> MSQEALKAPVVVLGAGLASVSFVAELRQAGYQGLITVVGDEAERPYDRPPLSKDFMAHGDAEKIRLDCKRAPEVEWLLGVTAQSFDPQAHTVALSDGRTLPYGTLVLATGAAPRALPTLQGATMPVHTLRTLEDARRIQAGLRPQSRLLIVGGGVIGLELAATARTAGVHVSLVQTKPRLMSRAAPATLADFVARYHAAQGVDLRFERSVTGSVDGVVLLDDGTRIAADMVVVGIGVLANDALARAAGLACDDGIFVDAYGRTTCPDVYALGDVTRQRNPLSGRFERIETWSNAQNQGIAVARHLVDPTAPGYAELPWYWSDQGALR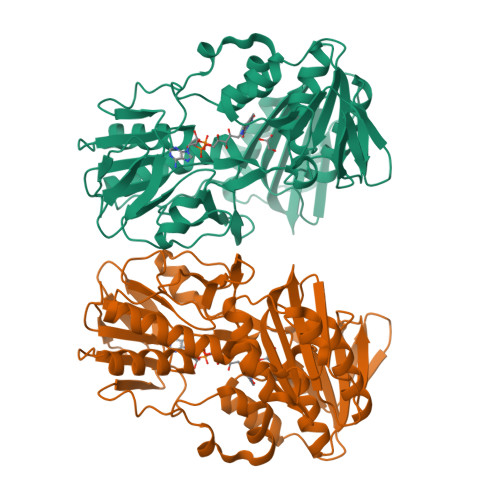IQVAGLASGDEEIVRGEVSLDAPKFTLIELQKGRIVGATCVNNARDFAPLRRLLAVGAKPDRAALADPATDLRKLAAAVAA>GANSVLFPCKYASSGCEITLPHTEKADHEELCEFRPYSCPCPGASCKWQGSLDAVMPHLMHQHKSITTLQGEDIVFLATDINLPGAVDWVMMQSCFGFHFMLVLEKQEKYDGHQQFFAIVQLIGTRKQAENFAYRLELNGHRRRLTWEATPRSIHEGIATAIMNSDCLVFDTSIAQLFAENGNLGINVTISMC[2x];>[2x]SPKPT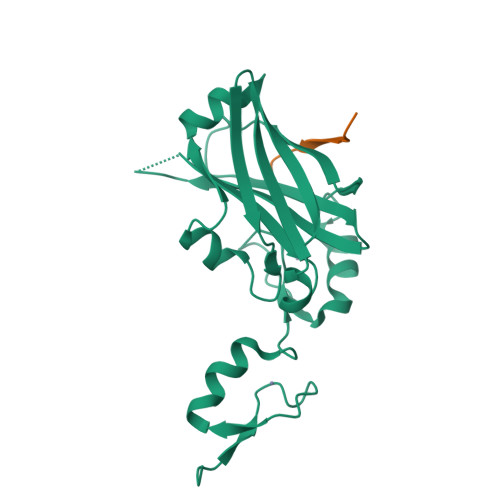CMVPPMPHS Prolidase Deficiency (PD) is an autosomal recessive rare disorder caused by loss or reduction of prolidase enzymatic activity due to variants in the PEPD gene. The PEPD gene encodes the enzyme peptidase D (EC 3.4.13.9), also known as prolidase, which is the only enzyme in humans capable of hydrolysis of dipeptides containing proline (Pro) or hydroxyproline (Hyp) on their C-terminus. Prolidase is particularly important in the degradation of collagens, a family of proteins where proline and hydroxyproline account for up to 22% of the amino acid content. We presented here two high-resolution crystal structures for the p.(Arg470His) variant of human prolidase.

The electron density maps clearly indicated the presence of an imidazol side chain rather than a guanidinum group at amino acid position 470, proving the success of the introduced amino acid substitution. In addition, comparison of structure of hProlArg470His to previously reported structure of hProl using Root Mean Square Deviation of Cα positions approach shows rather small structural differences mainly concentrated around poorly ordered C-termini. The only noticeable difference was the mutated residue. In hProl, Arg470 was located close to the active site and it formed hydrogen bond/ salt bridges with 3 residues: Thr289, Glu452 and Glu453. Glu452 is part of the active site and it participates in catalysis by coordinating both manganese ions. In case of hProlArg470His, substitution of Arg by His resulted in lesser number of salt bridges. His470 forms interacted only with Thr289 and Glu453. When comparing hProlR470H structures to hProl slightly higher B-factors of the His atoms than for the Arg atoms can be observed. This effect is more pronounced in the substrate-free structure. Based on our analysis we can classify the hProlArg470His variant of human prolidase as “structurally silent” and assume that loss of function of this particular mutant can arise from flexibilization of the active site.

>[2x]MAAATGPSFWLGNETLKVPLALFALNRQRLCERLRKNPAVQAGSIVVLQGGEETQRYCTDTGVLFRQESFFHWAFGVTEPGCYGVIDVDTGKSTLFVPRLPASHATWMGKIHSKEHFKEKYAVDDVQYVDEIASVLTSQKPSVLLTLRGVNTDSGSVCREASFDGISKFEVNNTILHPEIVECRVFKTDMELEVLRYTNKISSEAHREVMKAVKVGMKEYELESLFEHYCYSRGGMRHSSYTCICGSGENSAVLHYGHAGAPNDRTIQNGDMCLFDMGGEYYCFASDITCSFPANGKFTADQKAVYEAVLRSSRAVMGAMKPGVWWPDMHRLADRIHLEELAHMGILSGSVDAMVQAHLGAVFMPHGLGHFLGIDVHDVGGYPEGVERIDEPGLRSLRTARHLQPGMVLTVEPGIYFIDHLLDEALADPARASFLNREVLQRFRGFGGVRIEEDVVVTDSGIELLTCVPHTVEEIEACMAGCDKAFTPFSGPK>GPHMADPETAAKFKSKNAFPDPLNDPKCNPKSLVKKYLTPKVFESLKNKKTKLGITLWDCINSGVVNLDSGVGVYAGDEESYTLFGPLFDAIIEDYHSPYKLATGHNSDMNPAHVKAPDLDPANRYIRSTRIRVARSLKGYGLAPGVTKAHRLEIEKKVVGVLTSLTGDLAGKYYPLSGMDEKTRQQLVDDHFLFKKGDRFLEAAGINKEWPEGRGIYHNNDKTFLVWLNEEDHLRIISMEKGSDIGSVFSRLCRAVNEIDKKLGFQHTKKHGYLTSCPSNLGTGMRASVHVKIPHAKEHPDFENILTKYHIQARGIHGEHSESTGEDAGVYDISNRRRLGLSEVQCVQDMYDGVKALMELEKEAIAKKRSVFPEVLKNPEVKSLLRKYLTPELFDSLKDKKTAKGISLYDCINSGVENLDSSCGVYAGDEECYTLFAPLFDKIVEDYHSPYKLA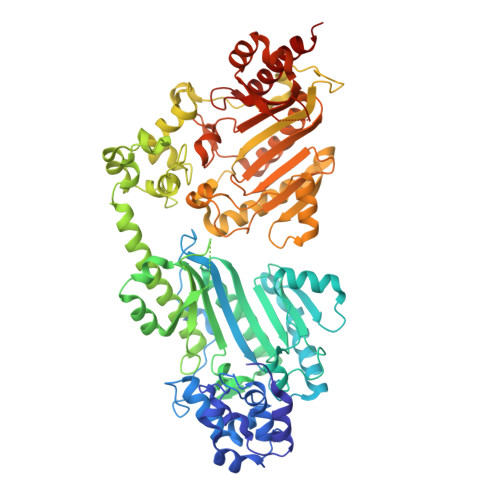NKHTSDMNPEKVDAPNLDPEGTYIRSTRIRVARNVKGYALTPGLTRNERLDIERKVVGVLSSLTGDLAGQYYPLTGMDEATRQKLVNDHFLFKKGDRFLEAAGVNKLWPEGRGIFHNNDKTFLVWINEEDQLRIISMEKGSDIGSVFGRLCRAVNEIDKQLGFQHTDAHGYLSGCPTNLGTGMRASVHVKIPKASAHPDFQKICDEFHIQARGIHGEHSVSTGEDAGVFDISNRRRLGLSEVQCVQDMYNGVKKLLEIEKSTK[2x]>[2x]GHMNKDNLRSPICCILGHVDTGKTKLLDKIRQTNVQ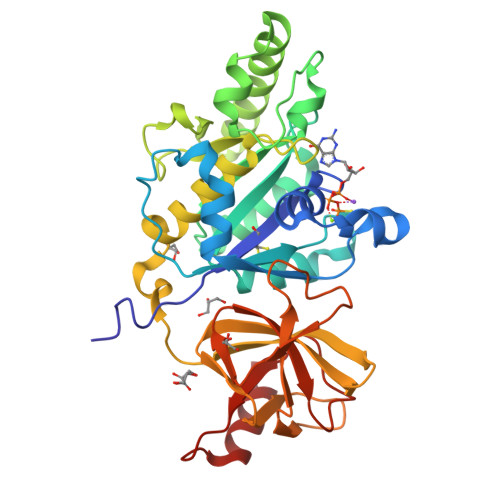EGEAGGITQQIGATYFPVEAIKQKTAVVNKDGKFEFKVPGLLIIDTPGHESFSNLRSRGSSLCNIAILVVDIMHGLEPQTIESLRLLRERKTPFVVALNKIDRLYGWKKIENNGFRESFALQNKAVQNEFRNRLDQVKLQFAEQGFNSELFYENKNFARYVSLVPTSAHTGEGIPDMLKLIVQLCQERMASSLMYLSELQATVLEVKAIEGFGVTIDVILSNGILREGDRIVLCGLEGPIKTNIRALLTPAPMRELRIKGQYIHHKEVKAAQGVKISAPGLEGAIAGSRLLVVGPDDDEEELEEEVESD>HHHHHHGGTILVVTGTGTGVGKTVVCAALASAARQAGIDVAVCKPVQTGTARGDDDLAEVGRLAGVTQLAGLARYPQPMAPAAAAEHAGMALPARDQIVRLIADLDRPGRLTLVEGAGGLLVELAEPGVTLRDVAVDVAAAALVVVTADLGTLNHTKLTLEALA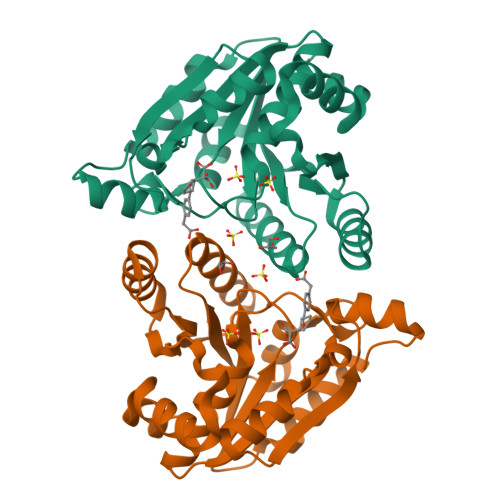AQQVSCAGLVIGSWPDPPGLVAASNRSALARIAMVRAALPAGAASLDAGDFAAMSAAAFDRNWVAGLVG[4x]> MKVAKDLVVSLAYQVRTEDGVLVDESPVSAPLDYLHGHGSLISGLETALEGHEVGDKFDVAVGANDAYGQYDENLVQRVPKDVFMGVDELQVGMRFLAETDQGPVPVEITAVEDDH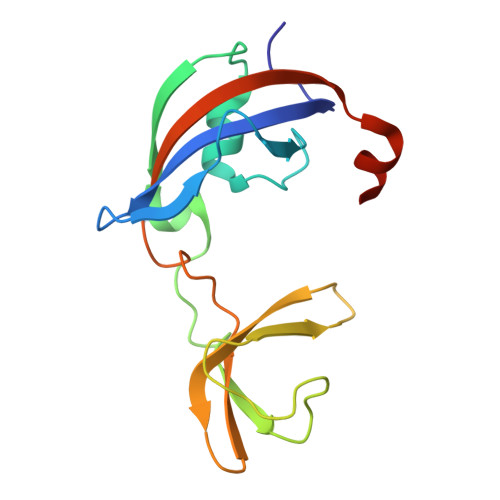VVVDGNHMLAGQNLKFNVEVVAIREATEEELAHGHVHG> GSMAQLGKLLKEQKYDRQLRLWGDHGQEALESAHVCLINATATGTEILKNLVLPGIGSFTIIDGNQVSGEDAGNNFFLQRSSIGKNRAEAAMEFLQELNSDVSGSFVEESPENLLDNDPSFFCRFTVVVATQLPESTSLRLADVLWNSQIPLLICRTYGLVGYMRIIIKEHPVIESHPDNALEDLRLDKPFPELREHFQSYDLDHMEKKDHSHTPWIVIIAKYLAQWYSETNGRIPKTYKEKEDFRDLIRQGILKPEDEENFEEAIKNVNTALNTTQIPSSIEDIFNDDRCINITKQTPSFWILARALKEFVAKEGQGNLPVRGTIPDMIADSGKYIKLQNVYREKAKKDAAAVGNHVAKLLQSIGQAPESISEKELKLLCS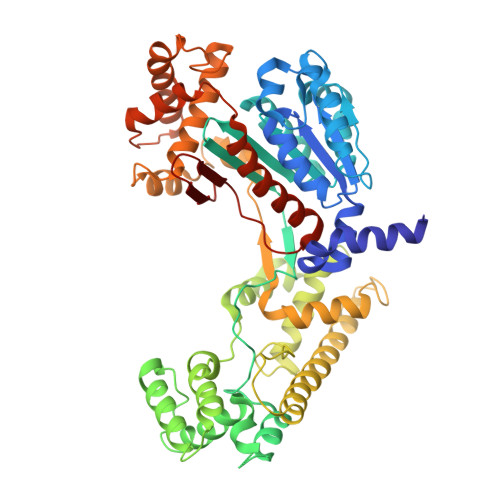NSAFLRVVRCRSLAEEYGLDTINKDEIISSMDNPDNEIVLYLMLRAVDRFHKQQGRYPGVSNYQVEEDIGKLKSCLTGFLQEYGLSVMVKDDYVHEFCRYGAAEPHTIAAFLGGAAAQEVIKIITKQFVIFNNTYIYSGMSQTSATFQL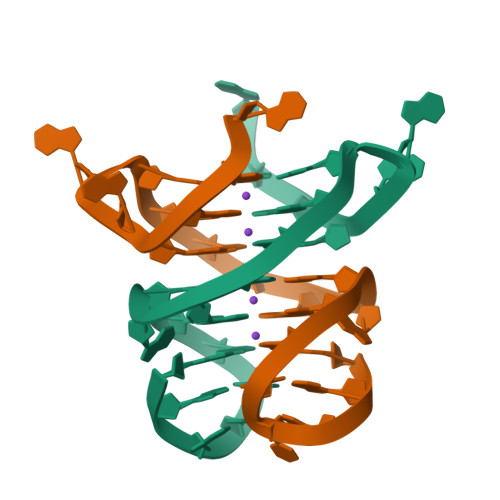>GGGCGGGGAGGGGGAAGGGA[2x]>MRIILLGAPGAGKGTQAQFIMEKYGIPQISTGDMLRAAVKSGSELGKQAKDIMDACKLVTDELVIALVKERIAQEDCRNGFLLDGFPRTIPQADAMKEAGINVDYVLEFDVPDELIVDRIVGRRVHAPSGRVYHVKFNPPKVEGKDDVTGEELTTR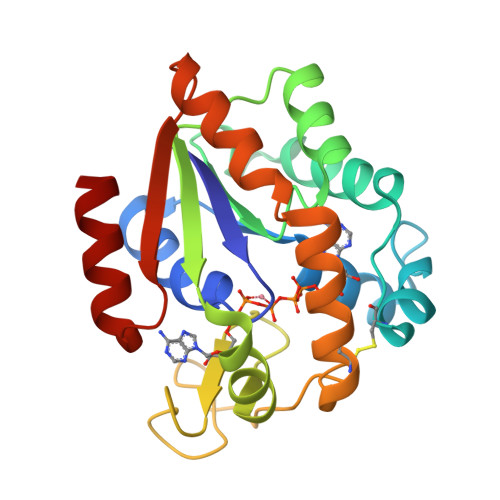KDDQEECVRKRLVEYHQMTAPLIGYYSKEAEAGNTKYAKVDGTKPVAEVRADLEKILG[2x]>MSQSGEDLHSPTYLSWRKLQLSRAKLKASSKTSALLSGFAMVAMVEVQLDHDTNVPPGMLIAFAICTTLLVAVHMLALMISTCILPNIETVSNLHSISLVHESPHERLHWYIETAWAFSTLLGLILFLLEIAILCWVKFYDLSPPAAWSATVV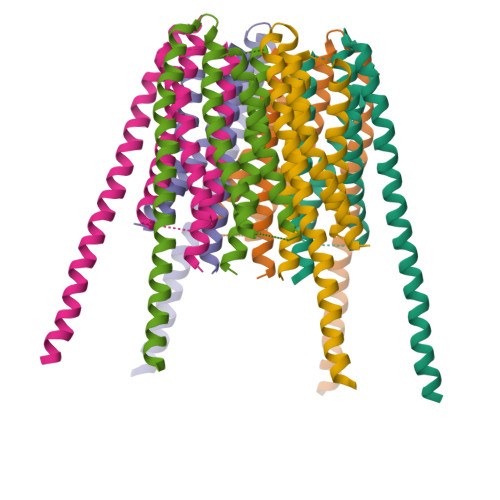LIPVMIIFMAFAIHFYRSLVSHKYEVTVSGIRELEMLKEQMEQDHLEHHNNIRNNGEGEEF[24x]>MTQTTQSPALIASQSSWRCVQAHDREGWLALMADDVVIEDPIGKSVTNPDGSGIKGKEAVG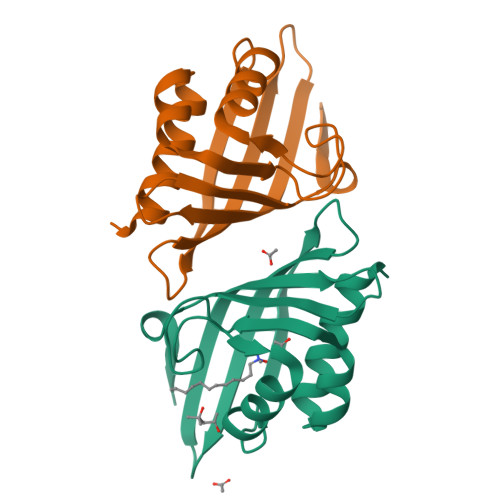AFFDTHIAANRLTVTCEETFPSSSPDEIAHILVLHSEFDGGFTSEVRGVFTYRVNKAGLITNMRGYWNLDMMTFGNQE[2x]> ET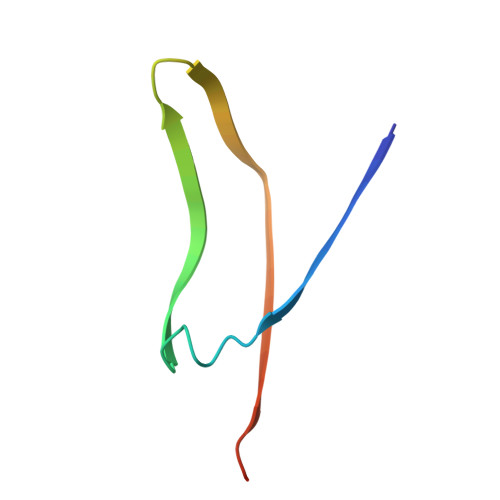SYTLNEVVPLKEFVPEWVRIGFSATTGAEFAAHEVLSWYFNSELSVTSSSN> MRNLKLHRTLEFRDIQAPGKPQCFCLRAEQGTVLIGSERGLTEVDPVRREVKTEISLVAEGFLPEDGSGCIVGIQDLLDQESVCVATASGDVIVCNLSTQQLECVGSVASGISVMSWSPDQELLLLATAQQTLIMMTKDFEVIAEEQIHQDDFGEGKFVTVGWGSKQTQFHGSEGRPTAFPVQLPENALPWDDRRPHITWRGDGQYFAVSVVCRQTEARKIRVWNREFALQSTSESVPGLGPALAWKPSGSLIASTQDKPNQQDVVFFEKNGLLHGHFTLPFLKDEVKVNDLLWNADSSVLAIWLEDLPKEDSSTLKSYVQLWTVGNYHWYLKQSLPFSTTGKNQIVSLLWDPVTPCRLHVLCTGWRYLCCDWHWTTDRSSGNSANDLANVAVIDGNRVLVTVFRQTVVPPPMCTYRLLIPHPVNQVIFSAHLGNDLAVLDASNQISVYKCGDKPNMDSTVKLGAVGGNGFKVPLTTPHLEKRYSIQFGNNEEEEEEEVNALQLSFLTWVEDDTFLAISYSHSSSQSIIHHLTVTHSEVDEEQGQLDVSSSVTVDGVVIGLCCCSKTKSLAVQLADGQVLKYLWESPSLAVEPWKNS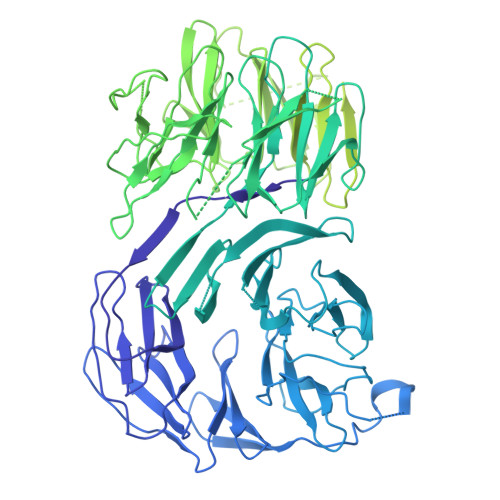EGIPVRFVHPCTQMEVATIGGEECVLGLTDRCRFFINDTEVASNITSFAVCDDFLLVTTHSHTCQVFSLSGASLKMLQAALSGSHEASGEILRKVERGSRIVTVVPQDTKLILQMPRGNLEVVHHRALVLAQIRKWLDKLMFKEAFECMRKLRINLNLIHDHNPKVFLENVETFVKQIDSVNHINLFFTELREEDVTKTMYPPPITKSVQVSTHPDGKKLDLICDAMRAAMEAINPRKFCLSILTSHVKKTTPELEIVLQKVQELQGNLPFDPESVSVEEALKYLLLLVDVNELFNHSLGTYDFNLVLMVAEKSQKDPKEYLPFLNTLKKMETNYQRFTIDKYLKRYEKALGHLSKCGPEYFTECLNLIKDKNLYKEALKLYRPDSPQYQAVSMAYGEHLMQEHLYEPAGLVFARCGAQEKALEAFLACGSWQQALCVAAQLQMSKDKVAGLARTLAGKLVEQRKHSEAATVLEQYAQDYEEAVLLLLEGSAWEEALRLVYKYDRVDIIETSVKPSILEAQKNYMDFLDSETATFIRHKNRLQVVRALRRQAPQVHVDHEVAHGPESDLFSETSSIMSGSEMSGRYSHSNSRISARSSKNRRKAERKKHSLKEGSPLEGLALLEALSEVVQSVEKLKDEVRAILKVLFLFEFEEQAKELQRAFESTLQLMERAVPEIWTPAGQQSSTTPVLGPSSTANSITASYQQQKTCVPALDAGVYMPPKMDPRSQWKLSLLE ethyl 3-methyl-4-{[4-(trifluoromethyl)-1,3-benzoxazol-7-yl]methyl}-1H-pyrrole-2-carboxylate 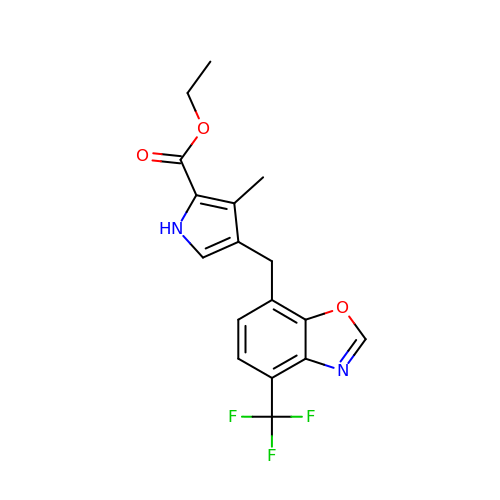| C17 H15 F3 N2 O3 | ZZBNHKLWSWWKKF-UHFFFAOYSA-N> MSAKKIVLKSSDGESFEVEEAVALESQTIAHMVEDDCVDN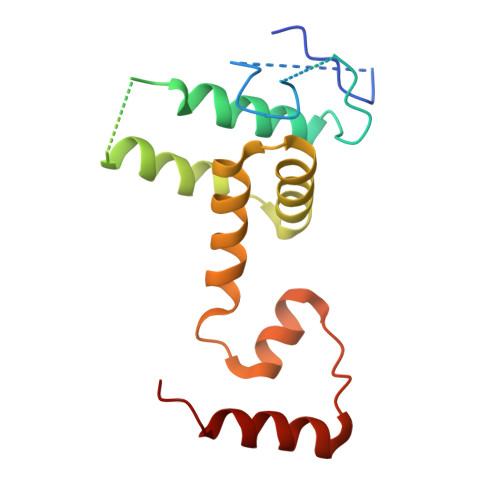GVPLPNVTSKILAKVIEYCKRHVEAAASKAEAVEGAATSDDDLKAWDADFMKIDQATLFELILAANYLNIKNLLDLTCQTVADMIKGKTPEEIRTTFNIKNDFTPEEEEEVRRENQWAFE> XEVEALEKKV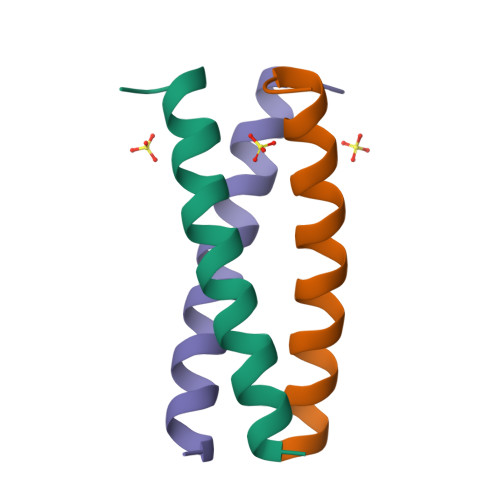AALESKVQALEKKVEALEHGX>SNAMKVTQLSSETLDRAHERFEETLAQMTVAEANTMPAPLIKSVTWLMWHTARELDLQISALNHSDPLWLSQHWTEKFALDLPDETEDWHHTPEEAAKVVVAEKQLLSDYLAASVALTKSYLDQIKEEQLSDVIDKNWTPPVTRQVRLVSAIDDA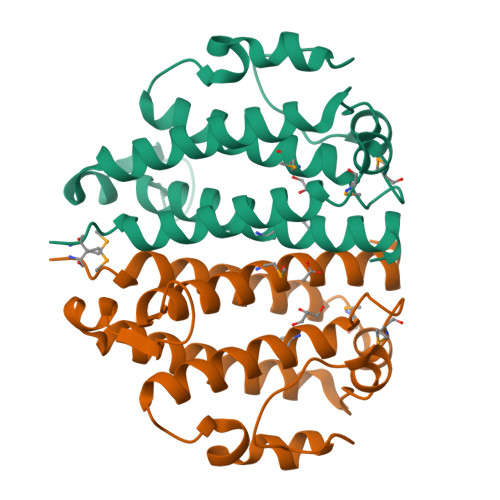VMHSGQAVYTRRLVIGK[2x]> IHEGPYPEPLVNL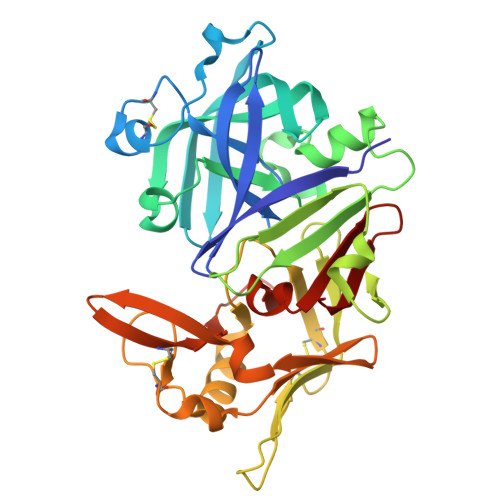LDVVYYGPISIGTPPQDFQVIFDTGSANLWLPSSKCTTKYCLHHHRYDSSKSSTYEADGRNFTIVYGSGNVEGFISKDVCRIGSAKVSGQPLGEALVVGGESLLEAPFDGILGLAYPSIAVDGVVPVFDNMMKQGLLGEQNVFSVYLNRDPSSKEGGEVLFGGIDHDHYKGSITYVPVTAKGYWQFHVDGVKSVSASKSAPELLCKDGCEAIADTGTSLITGPPEEVDSLNQYLGGTKTEGGQYLLDCDKLESLPNVTFTISGKEFSLRSKDYVLKVNQQGQTLCVSGFMGLEMPQPLWILGDVFLGPYYTIFDRDQDRVGFAEVA> NAKTSTKVKQMMDLTFDLATPIDKRRAAANNLVVLAKEQTGAELLYKDHCIAKVASLTKVEKDQDIYVNMVHLVAALCENSVERTKGVLTELGVPWFMRVLDQKHENCVSTAQFCLQTILNALSGLKNKPDSKPDKELCTRNNREIDTLLTCLVYSITDRTISGAARDGVIELITRNVHYTALEWAERLVEIRGLCRLLDVCSELEDYKYESAMDITGSSSTIASVCLARIYENMYYDEAKARFTDQIDEYIKDKLLAPDMESKVRVTVAITALLNGPLDVGNQVVAREGILQMILAMATTDDELQQRVACECLIAASSKKDKAKALCEQGVDILKRLYHSKNDGIRVRALVGLCKLGSYGGQDAAIRPFGDGAALKLAEACRRFLIKPGKDKDIRRWAADGLAYLTLDAECKEKLIEDKASIHALMDLARGGNQSCLYGVVTTFVNLCNAYEKQEMLPEMIELAKFAKQHIPEEHELDDVDFINKRITVLANEGITTALCALAKTESHNSQELIARVLNAVCGLKELRGKVVQEGGVKALLRMALEGTEKGKRHATQALARIGITINPEVSFSGQR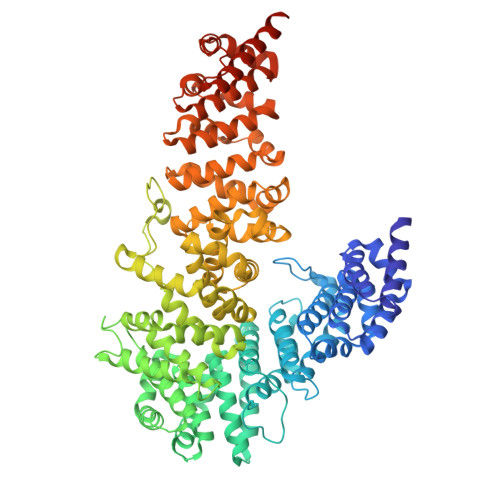SLDVIRPLLNLLQQDCTALENFESLMALTNLASMNESVRQRIIKEQGVSKIEYYLMEDHLYLTRAAAQCLCNLVMSEDVIKMFEGNNDRVKFLALLCEDEDEETATACAGALAIITSVSVKCCEKILAIASWLDILHTLIANPSPAVQHRGIVIILNMINAGEEIAKKLFETDIMELLSGLGQLPDDTRAKAREVATQCLAAAERYRIIERSDNAEIPDVFAENSKISEIIDD~{N}-~{tert}-butyl-9,10-bis(oxidanylidene)anthracene-2-sulfonamide | C18 H17 N O4 S 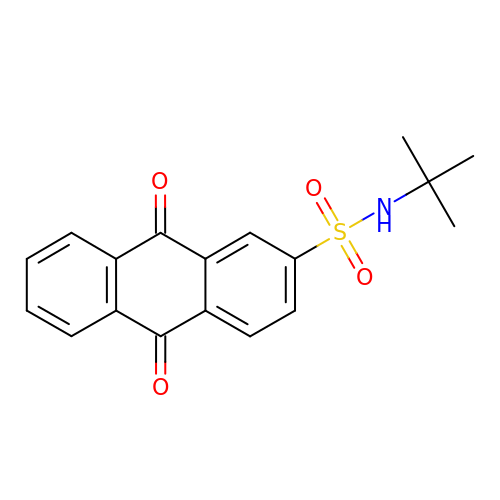| LWNJBYGFPRLQHH-UHFFFAOYSA-N> TGAEPQALPSDPLEQALHQAWQAQLGAPPRAGQGFYAAGGDSLRAVHLLATLRQRLSRRVPLQAFAGGPATPEALLELLRQAAPEGDEPEPSAGAAGLSLAERRLWVAQQLAPEDTSYNLLAHLRIVGATADAIEQALRQLLERHVALRRRVETGVDGPQPHALAAHAVPLQRLLASDAVHAERLLEDGVRREGARVFDLAHEAPARLLLVVTRDSARADLLLSVHHYAFDDVSLAVFAAELKTLLDGGRLGVLASTPEQVAARERAALASGRLDRVAERWAERLLPLAKAPGAAPARPEESGGRAGQRLALPVSAAVHAACRALAERTSVSPFSAALQAFAEVLGAELGVDDLLVGVALAGRSRLEMQGLVGCFVNLLPLAVGLRPEQSVEWRLRQVGHDLLELLEHQDVPLECVTQALRQRGASGLPIRIACGAHNGRAAPAVDAGVRVEADFIPVPGARLDLTLWLEDQPQGWLAVWTGVSA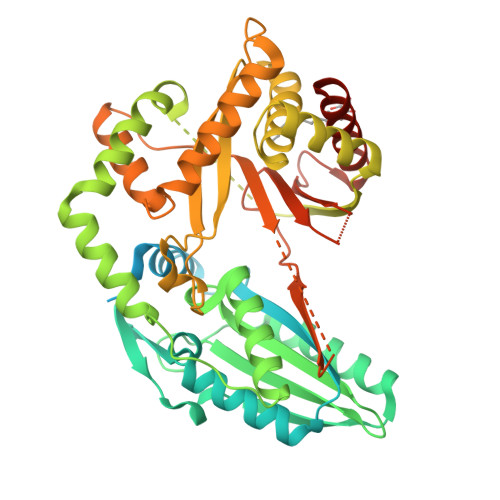IFDLHRIERLHQAWERRLLANAGEPISKRMSPEGCNAS> 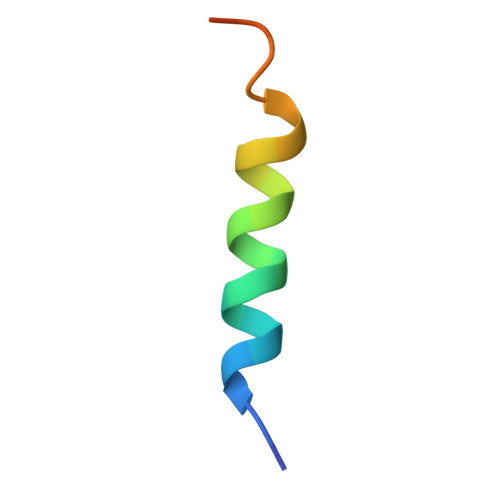HQAEVQIARKLQCIADQFHRLHVQQ>SHMASMPPYTVVYFPVRGRCAALRMLLADQGQSWKEEVVTVETWQEGSLKASCLYGQLPKFQDGDLTLYQSNTILRHLGRTLGLYGKDQQEAALVDMVNDGVEDLRCKYISLIYTNYEAGKDDYVKALPGQLKPFETLLSQNQGGKTFIVGDQISFADYNLLDLLLIHEVLAPGCLDAFPLLSAYVGRLSARPKLKAFLASPEYVNLPINGNGKQ[2x]

Since NQO1 and GSTP1 are phase-II detoxification enzymes that reduce quinones directly to hydroquinones, eliminating the formation of ROS produced by redox cycling, the combination of inhibition of NQO1 and GSTP1 may offer a potential solution for cancer therapy. Though previous studies demonstrate the importance of NQO1 signaling for the progressive phenotype in colorectal cancer and GSTP1 is overexpressed in many cancers and linked to drug resistance, the molecular mechanisms of how these reductive enzymes involved in GBM proliferation remain unclear. Both NQO1 and GSTP1 are well-known phase II metabolism enzymes catalyzing diverse reactions that collectively result in broad protection against electrophiles and oxidants. Using a strategy based on high-throughput chemical screening (HTS) and affinity chromatography, we identified a small molecule NQO1 and GSTP1 dual inhibitor, MNPC, that suppressed the proliferation and stimulated apoptosis in a highly passaged cell line and primary GBM cells bearing the EGFRvIII mutation. The co-crystal structure between MNPC and NQO1, and the molecular docking of MNPC with GSTP1 revealed that MNPC blocked the active sites in both enzymes.

Glutathione S-transferases (GSTs) catalyze reactions between glutathione and lipophilic compounds with electrophilic centers, leading to the neutralization of toxic compounds, xenobiotics and products of oxidative stress. Attempts at co-crystallization between MNPC with GSTP1 revealed some electron density in the putative inhibitor binding site. However, it could not be fitted for the whole MNPC molecule. Therefore, we performed the molecular docking and subsequent mutagenesis analysis to elucidate the binding mode of MNPC with GSTP1. From the generated docking model, we found that MNPC was located in the active pocket of GSTP1, closely adjacent to the substrate GSH. It formed two hydrogen bindings with Arg100 and Tyr108 and one hydrogen bonding with GSH. MNPC also exhibited the π-π stacking with Phe8 and Tyr108. To further verify the docking results, site-directed mutagenesis was conducted to generate several mutants (F8A, R100A, V104A, Y108A, F8A/Y108A), and inhibition of enzymatic activity against these mutants was measured. Importantly, the inhibition of MNPC decreased the most with Y108A mutant, which was consistent with the docking results that Tyr108 formed both hydrogen bonding and hydrophobic interaction with MNPC. Taken together, the data show that Tyr108 is the most important amino acid for binding of GSTP1 with MNPC, while Phe8 and Arg100 also participate in the interaction between MNPC and GSTP1.>MGSHHHHHHENLYFQGHMNSFYSQEELKKIGFLSVGKNVLISKKASIYNPGVISIGNNVRIDDFCILSGKVTIGSYSHIAAYTALYGGEVGIEMYDFANISSRTIVYAAINDFSGNALMGPTIPNQYKNVKTGKVILKKHVIIGAHSIIFPNVVIGEGVAVGAMSMVKESLDDWYIYVGVPVRKIKARKRKIVELENEFL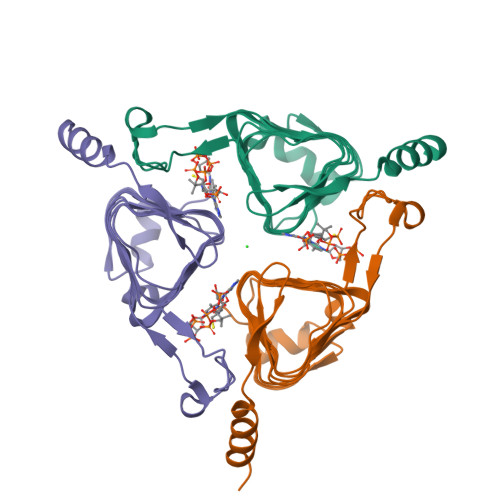KSMNS[3x]N-[[1-[[2-[3,5-bis(chloranyl)phenyl]-6-[6-[4-(2-methoxyethyl)piperazin-4-ium-1-yl]pyridin-3-yl]oxy-pyridin-4-yl]methyl]piperidin-1-ium-4-yl]methyl]ethanamide 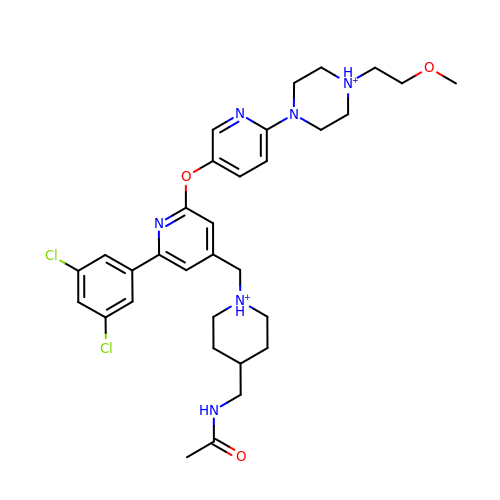| C32 H42 Cl2 N6 O3 | AUPHEGBHBGKBKL-UHFFFAOYSA-P> MFGLIGHLTSLEQARDVSRRMGYDEYADQGLEFWSSAPPQIVDEITVTSATGKVIHGRYIESCFLPEMLAARRFKTATRKVLNAMS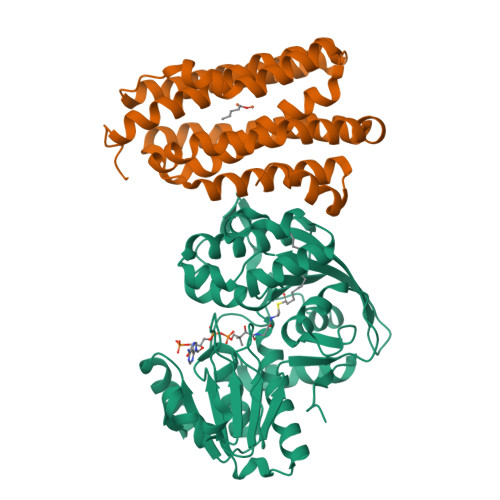HAQKHGIDISALGGFTSIIFENFDLASLRQVRDTTLEFERFTTGNTHTAYVICRQVEAAAKTLGIDITQATVAVVGATGDIGSAVCRWLDLKLGVGDLILTARNQERLDNLQAELGRGKILPLEAALPEADFIVWVASMPQGVVIDPATLKQPCVLIDGGYPKNLGSKVQGEGIYVLNGGVVEHCFDIDWQIMSAAEMARPERQMFASFAEAMLLEFEGWHTNFSWGRNQITIEKMEAIGEASVRHGFQPLALAI;> MRTPWDPPNPTFSLSSVSGDRRLMPQLEASLELDFQSESYKDAYSRINAIVIEGEQEAFDNYNRLAEMLPDQRDELHKLAKMEQRHMKGFMACGKNLSVTPDMGFAQKFFERLHENFKAAAAEGKVVTCLLIQSLIIECFAIAAYNIYIPVADAFARKITEGVVRDEYLHRNFGEEWLKANFDASKAELEEANRQNLPLVWLMLNEVADDARELGMERESLVEDFMIAYGEALENIGFTTREIMRMSAYGLAAV>[2x]GPDSMPIDWTIEEVIQYIESNDNSLAVHGDLFRKHEIDGKALLLLNSEMMMKYMGLKEGPAEKICNLVNKVNGRR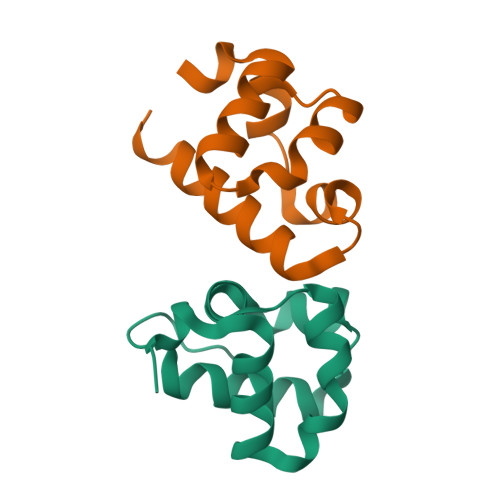NNLAL;>[2x]GPDSMPDTWNVYDVSQFLRVNDCTAHCDTFSRNKIDGKRLLQLTKDDIMPLLGMKVGPALKISDLIAQLKCKVNPGRARSHKTNKSPFL>[4x]MSREVFICDAVRTPIGRFGGSLSAVRADDLAAVPLKALVERNPGVDWSALDEVFLGCANQAGEDNRNVARMALLLAGLPESVPGVTLNRLCASGMDAIGTAFRAIACGEMELAIAGGVESMSRAPYVMGKADSAFGRGQKIEDTTIGWRFVNPLMKEQYGIDPMPQTADNVADDYRVSRADQDAFALRSQQRAGRAQE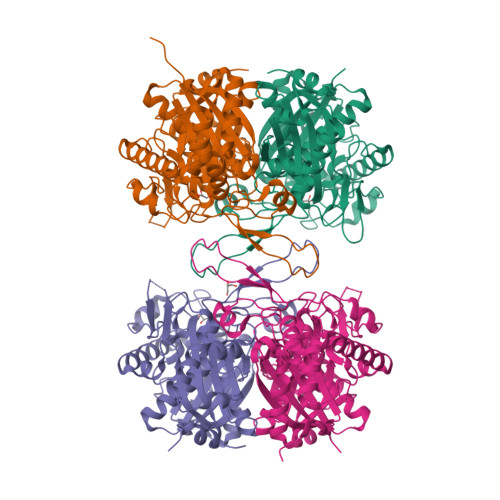AGFFAEEIVPVTIRGRKGDTLVEHDEHPRPDTTLEALARLKPVNGPEKTVTAGNASGVNDGAAALVLASAEAVEKHGLTPRARVLGMASAGVAPRIMGIGPVPAVRKLLRRLDLAIDAFDVIELNEAFASQGLACLRELGVADDSEKVNPNGGAIALGHPLGMSGARLVLTALHQLEKSGGRRGLATMCVGVGQGLALAIERVLEHHHHHH> EPQNCSA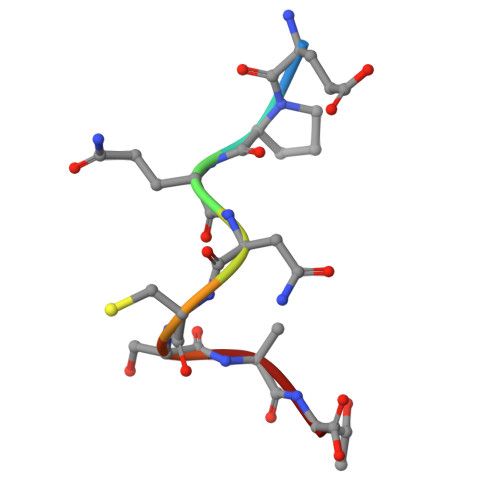T>[3x]MLAKRIIACLNVKDGRVVKGTNFENLRDSGDPVELGKFYSEIGIDELVFLDITASVEKRKTMLELVEKVAEQIDIPFTVGGGIHDFETASELILRGADKVSINTAAVENPSLITQIAQTFGSQAVVVAIDAKRVDGEFMVFTYSGKKNTGILLRDWVVEVEKRGAGEILLTS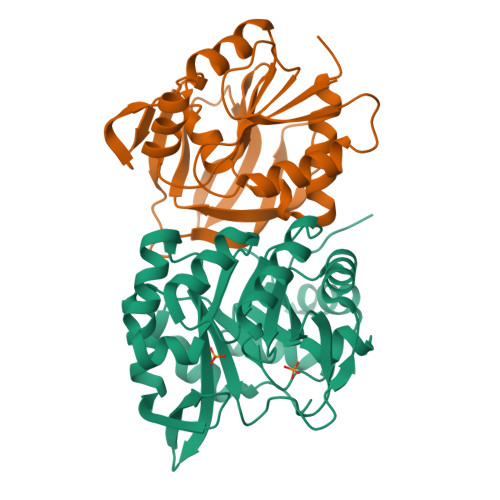IDRDGTKSGYDTEMIRFVRPLTTLPIIASGGAGKMEHFLEAFLAGADAALAASVFHFREIDVRELKEYLKKHGVNVRLEGL;>[3x]MRIGIISVGPGNIMNLYRGVKRASENFEDVSIELVESPRNDLYDLLFIPGVGHFGEGMRRLRENDLIDFVRKHVEDERYVVGVCLGMQLLFEESEEAPGVKGLSLIEGNVVKLRSRRLPHMGWNEVIFKDTFPNGYYYFVHTYRAVCEEEHVLGTTEYDGEIFPSAVRKGRILGFQFHPEKSSKIGRKLLEKVIECSLSRR>[2x]GSHMRFDEFGNIITDSAVAEEPEPELPGVTEEALRLKEAALEELAAQEVTAPLVPLAVSAFLTSRKKAAAAELADWMQSPEGQASSLESIGRSLSRRNHGRSRAVVLAHDHDEAIKGLR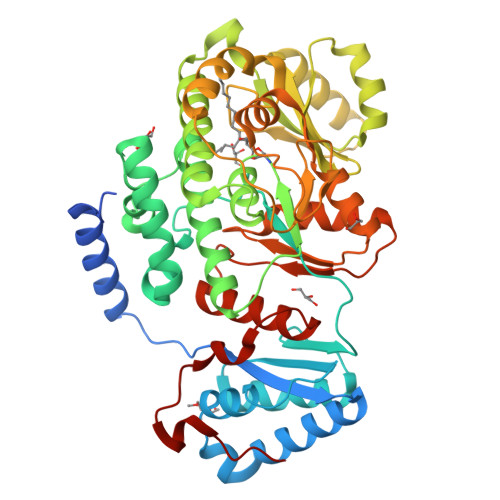AVAAGKQAPNVFSVDGPVTTGPVWVLAGFGAQHRKMGKSLYLRNEVFAAWIEKVDALVQDELGYSVLELILDDAQDYGIETTQVTIFAIQIALGELLRHHGAKPAAVIGQSLGEAASAYFAGGLSLRDATRAICSRSHLMGEGEAMLFGEYIRLMALVEYSADEIREVFSDFPDLEVCVYAAPTQTVIGGPPEQVDAILARAEAEGKFARKFATKGASHTSQMDPLLGELTAELQGIKPTSPTCGIFSTVHEGRYIKPGGEPIHDVEYWKKGLRHSVYFTHGIRNAVDSGHTTFLELAPNPVALMQVALTTADAGLHDAQLIPTLARKQDEVSSMVSTMAQLYVYGHDLDIRTLFSRASGPQDYANIPPTRF;> SDKENFWGMAVA>QEQVAPPKDPAAALEDHKTRTDNRSEPSLDNLAQQDVAAPGAPEGVSALSDAQYNEANKIYFERCAGCHGVLRKGATGKALTPDLTRDLGFDYLQSFITYGSPAGMPNWGTSGELSAEQVDLMANYLLLDPAAPPEFGMKEMRESWKVHVAPEDRPTQQENDWDLENLFSVTLRDAGQIALID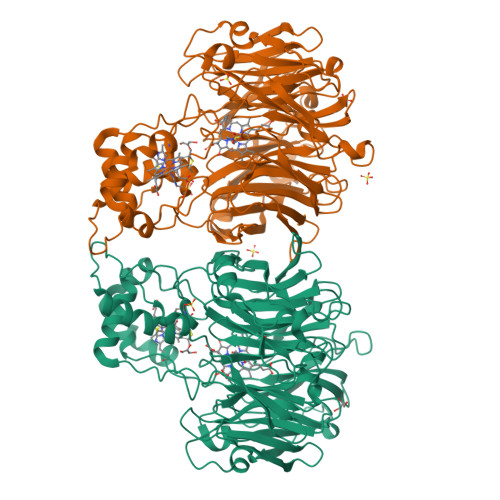GATYEIKSVLDTGYAVHISRLSASGRYLFVIGRDGKVNMIDLWMKEPTTVAEIKIGSEARSIETSKMEGWEDKYAIAGAYWPPQYVIMDGETLEPKKIQSTRGMTYDEQEYHPEPRVAAILASHYRPEFIVNVKETGKILLVDYTDLDNLKTTEISAERFLHDGGLDGSHRYFITAANARNKLVVIDTKEGKLVAIEDTGGQTPHPGRGANFVHPTFGPVWATSHMGDDSVALIGTDPEGHPDNAWKILDSFPALGGGSLFIKTHPNSQYLYVDATLNPEAEISGSVAVFDIKAMTGDGSDPEFKTLPIAEWAGITEGQPRVVQGEFNKDGTEVWFSVWNGKDQESALVVVDDKTLELKHVIKDERLVTPTGKFNVYNTMTDTY[2x]> MLGIRSSVKTCFKPMSLTSKRLISQSLLASKSTYRTPNFDDVLKENNDADKGRSYAYFMVGAMGLLSSAGAKSTVETFISSMTATADVLAMAKVEV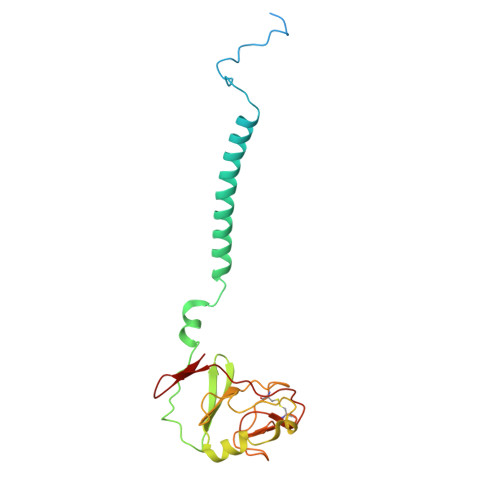NLAAIPLGKNVVVKWQGKPVFIRHRTPHEIQEANSVDMSALKDPQTDADRVKDPQWLIMLGICTHLGCVPIGEAGDFGGWFCPCHGSHYDISGRIRKGPAPLNLEIPAYEFDGDKVIVG> MGTHYKLGSDISQKSIPKEVKVAIVGAGMSGLYSAWRLQSEANVGDLAIFERSDRTGGRLDSDLIEFKDNRAGAEPGSTITVKEEQGGMRFL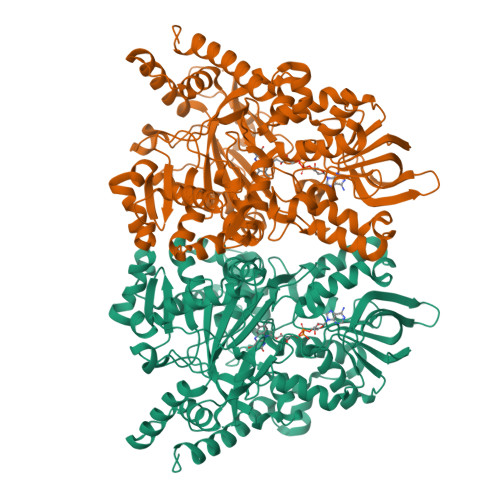FEGMDDLMALFLKLGLEDQIVPFPMNSGGNNRLYFRGTSFSVNDAEQDDYHIWSALYNLDPSEQGVNPKDIINVVFNRILQVNPQFDSRPEVRGPEFWQNFRLQCQWQGEPLYNWSLWDLLTDMGYSQECITMLYRVLGFNGTFLSKMNAGVAYQLLEDFPADVEFRTFKDGFSTLPNALVDKIGKDKIHLQTSIDSIAFDKADSKYVLKYTKIDQSGQVSEGKFKAEKVILGLPRLALEKLFIASDAFKQLPKKRRDELWDTLQSTSNQPLLKINLYYDTAWWGTGMTGRPAVSFGPNFADLPTGSVYPFYALNDELAAALMYDERHATPNPDTQHKLDGIDAAKYARPAALTIYCDYLNINFWSALQNKGELYHHPHESELVESIPSDIFPASEAVVQQATQFFKDIFNTHYVPQPTLTSARIWEGNVNFNVPENLQFGFGVHQWAIGANDKEVIEDLVEPLPNLFTCGEAYSDYQGWVEGALRSTDLVLQKGFGLAPLSEVYEQDQGRSSSEAIQIAYRKISNKMIMEYIDPNFSPNTKHKVTLAEVNSVLGVNLSYFDKPEHHHHHH> GHMSQHLPLVAAQPGIWMAEKLSELPSAWSVAHYVELTGEVDSPLLARAVVAGLAQADTLRMRFTEDNGEVWQWVDDALTFELPEIIDLRTNIDPHGTAQALMQADLQQDLRVDSGKPLVFHQLIQVADNRWYWYQRYHHLLVDGFSFPAITRQIANIYCTWLRGEPTPASPFTPFADVVEEYQQYRESEAWQRDAAFWAEQRRQLPPPASLSPAPLPGRSASADILRLKLEFTDGEFRQLATQLSGVQRTDLALALAALWLGRLCNRMDYAAGFIFMRRLGSAALTATGPVLNVLPLGIHIAAQETLPELATRLAAQLKKMRRHQRYDAEQIVRDSGRAAGDEPLFGPVLNIKVFDYQLDIPDVQAQTHTLATGPVNDLELALFPDVHGDLSIEILANKQRYDEPTLIQHAERLKMLIAQFAADPALLCGDVDIMLPGEYAQLAQLNATQVEIPETTLSALVAEQAAKTPDAPALADARYLFSYREMREQVVALANLLRERGVKPGDSVAVALPRSVFLTLALHAIVEAGAAWLPLDTGYPDDRLKMMLEDARPSLLITT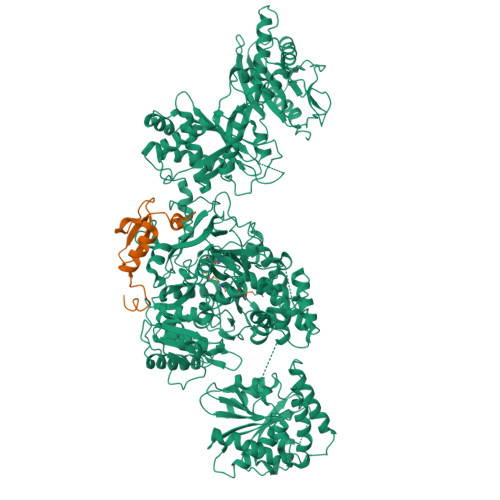DDQLPRFSDVPNLTSLCYNAPLTPQGSAPLQLSQPHHTAYIIFTSGSTGRPKGVMVGQTAIVNRLLWMQNHYPLTGEDVVAQKTPCSFDVSVWEFFWPFIAGAKLVMAEPEAHRDPLAMQQFFAEYGVTTTHFVPSMLAAFVASLTPQTARQSCATLKQVFCSGEALPADLCREWQQLTGAPLHNLYGPTEAAVDVSWYPAFGEELAQVRGSSVPIGYPVWNTGLRILDAMMHPVPPGVAGDLYLTGIQLAQGYLGRPDLTASRFIADPFAPGERMYRTGDVARWLDNGAVEYLGRSDDQLKIRGQRIELGEIDRVMQALPDVEQAVTHACVINQAAATGGDARQLVGYLVSQSGLPLDTSALQAQLRETLPPHMVPVVLLQLPQLPLSANGKLDRKALPLPELKAQAPGRAPKAGSETIIAAAFSSLLGCDVQDADADFFALGGHSLLAMKLAAQLSRQVARQVTPGQVMVASTVAKLATIIDAEEDSTRRMGFETILPLREGNGPTLFCFHPASGFAWQFSVLSRYLDPQWSIIGIQSPRPNGPMQTAANLDEVCEAHLATLLEQQPHGPYYLLGYSLGGTLAQGIAARLRARGEQVAFLGLLDTWPPETQNWQEKEANGLDPEVLAEINREREAFLAAQQGSTSTELFTTIEGNYADAVRLLTTAHSVPFDGKATLFVAERTLQEGMSPERAWSPWIAELDIYRQDCAHVDIISPGTFEKIGPIIRATLNR;> GHMAFSNPFDDPQGAFYILRNAQGQFSLWPQQCVLPAGWDIVCQPQSQASCQQWLEAHWRTLTPTNFTQLQEAQ> GCGGAUUUAGCUCAGUUGGGAGAGCGCCAGACUGAAGAUCUGGAGGUCCUGUGUUCGAUCCACAGAAUUC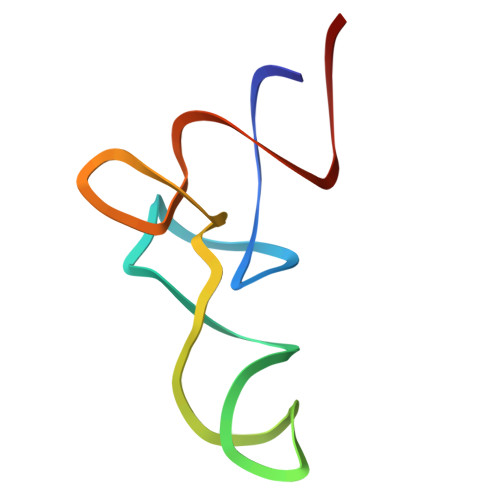GCACC>[2x]VNVVAGGPVANY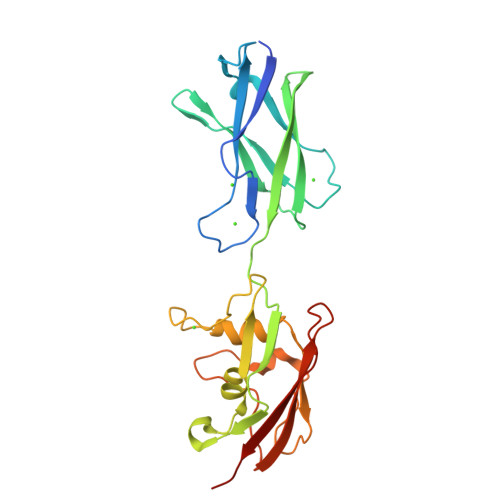QIKVLDDGKIDKSATESPANNDVQLKVYAVDANGNIVGDITNDVTITSEATDTNGVIVNASKSTANGDTVYVITDNGSKKVGKETLTVKLGTVTLGTVDVEVIDTTLKATVVTKKADLIELDAADNGDALAKLLANLDIKDQNGNPMVDSAATPNTNEKLQALKSVLSGIVSSDTSVIGSVSNVDNLKDDASISGLAVKKAGTVTLTLVFNEDSKIAPIAITVKAPAAT>GDEKDGPSKKILVTNAGVTEANQTVKPGDIVHIYGDGFQEGDQVDFDFRWDLGEPLFPEGYLGPVGAEIVERHSNGMSIRMPYRKPESRVEIFLNRASERMSLGKVLLADGQTPKDFRLYGINETDKTIERAYAEETVTGKKTWDMSAHPDFRSVVNLQKTYGLCGLAEENGVQQPFFLDFCTGEWKALSFYDYNTLALVIGSGNDIAAIQQRGKGYSLYNVSAGLEQSNYATKTRSNFPMPEPQFELPEGFTPEQFGDYPGVFMQGNEIILLSARKGNGKWVPMLYNYRNGFYVLEGIEADAIIPFYFGMALPDSGSPSLLYQKKVGYMIYYSSGDNRGSSFRLLEPDKESSKLQLQEPFAQLSDK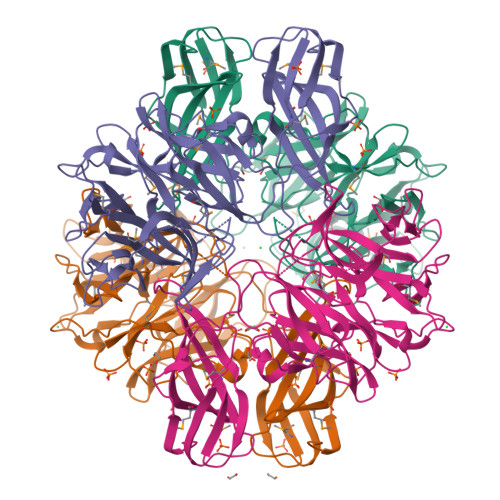KVVSITNRLDRIGTITVLFSDKEKGRTTSDFDWNSKEWTDYTDLSDMPYNSVVWAN[2x]>[2x]ADKLFINALKKKFEESPEEKKTTFYTLGGWKQSERKTEFVNAGKEVAAKRGIPQYNPDIGTPLGQRVLMPYQVSTTDTYVEGDDLHFVNNAAMQQMWDDIRRTVIVGLNHAHAVIEKRLGKEVTPETITHYLETVNHAMPGAAVVQEHMVETHPALVADSYVKVFTGNDEIADEIDPAFVIDINKQFPEDQAETLKAEVGDGIWQVVRIPTIVSRTCDGATTSRWSAMQIGMSMISAYKQAAGEAATGDFAYAAKHAEVIHMGTYLPVRRARGENEPGGVPFGYLADICQSSRVNYEDPVRVSLDVVATGAMLYDQIWLGSYMSGGVGFTQYATAAYTDNILDDFTYFGKEYVEDKYGLCEAPNNMDTVLDVATEVTFYGLEQYEEYPALLEDQFGGSQRAAVVAAAAGCSTAFATGNAQTGLSGWYLSMYLHKEQHSRLGFYGYDLQDQCGASNVFSIRGDEGLPLELRGPNYPNYAMNVGHQGEYAGISQAPHAARGDAFVFNPLVKIAFADDNLVFDFTNVRGEFAKGALREFEPAGERALITPAK;>[2x]AKFEDKVDLYDDRGNLVEEQVPLEALSPLRNPAIKSIVQGIKRTVAVNLEGIENALKTAKVGGPACKIMGRELDLDIVGNAESIAAAAKEMIQVTEDDDTNVELLGGGKRALVQVPSARFDVAAEYSAAPLVTATAFVQAIINEFDVSMYDANMVKAAVLGRYPQSVEYMGANIATMLDIPQKLEGPGYALRNIMVNHVVAATLKNTLQAAALSTILEQTAMFEMGDAVGAFERMHLLGLAYQGMNADNLVFDLVKANGKEGTVGSVIADLVERALEDGVIKVEKELTDYKVYGTDD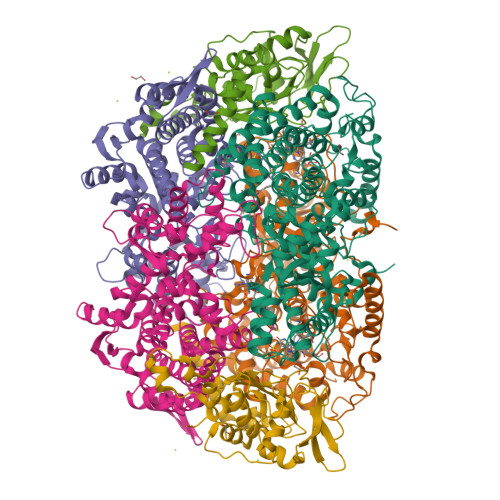LAMWNAYAAAGLMAATMVNQGAARAAQGVSSTLLYYNDLIEFETGLPSVDFGKVEGTAVGFSFFSHSIYGGGGPGIFNGNHIVTRHSKGFAIPCVAAAMALDAGTQMFSPEATSGLIKEVFSQVDEFREPLKYVVEAAAEIKNEI;>[2x]AQYYPGTTKVAQNRRNFCNPEYELEKLREISDEDVVKILGHRAPGEEYPSVHPPLEEMDEPEDAIREMVEPIDGAKAGDRVRYIQFTDSMYFAPAQPYVRSRAYLCRYRGADAGTLSGRQIIETRERDLEKISKELLETEFFDPARSGVRGKSVHGHSLRLDEDGMMFDMLRRQIYNKDTGRVEMVKNQIGDELDEPVDLGEPLDEETLMEKTTIYRVDGEAYRDDVEAVEIMQRIHVLRSQGGFNLE> GDPIADMIDQTVNNQVNRSLTALQVLPTAANTEASSHRLGTGVVPALQAAETGASSNASDKNLIETRCVLNHHSTQETAIGNFFSRAGLVSIITMPTTGTQNTDGYVNWDIDLMGYAQLRRKCELFTYMRFDAEFTFVVAKPNGELVPQLLQYMYVPPGAPKPTSRDSFAWQTATNPSV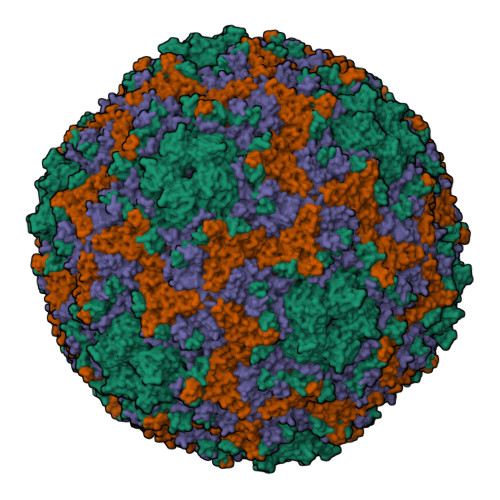FVKMTDPPAQVSVPFMSPASAYQWFYDGYPTFGEHLQANDLDYGQCPNNMMGTFSIRTVGIEKSPHSITLRVYMRIKHVRAWIPRPLRNQPYLFKTNPNYKGNDIKCTSTSRDKITTL;> SPSAEACGYSDRVAQLTIGNSTITTQEAANIVIAYGEWPEYCPDTDATAVDKPTRPDVSVNRFFTLDTKSWAKDSKGWYWKFPDVLTEVGVFGQNAQFHYLYRSGFCVHVQCNASKFHQGALLVAVLPEYVLGTIAGGTGNENSHPPYATTQPGQVGAVLTHPYVLDAGIPLSQLTVCPHQWINLRTNNCATIIVPYMNTVPFDSALNHCNFGLLVIPVVPLDFNTGATSEIPITVTIAPMCAEFAGLRQAVKQ;> GIPTELKPGTNQFLTTDDGVSAPILPGFHPTPPIHIPGEVHNLLEICRVETILEVNNLKTNETTPMQRLCFPVSVQSKTGELCAAFRADPGRDGPWQSTILGQLCRYYTQWSGSLEVTFMFAGSFMATGKMLIAYTPPGGNVPADRITAMLGTHVIWDFGLQSSVTLVVPWISNTHYRAHARAGYFDYYTTGIITIWYQTNYVVPIGAPTTAYIVALAAAQDNFTMKLCKDTEDIEQTANIQ;> MGSQVSTQRSGSHENSNSASEGSTINYTTINYYKDAYAASAGRQDMSQDPKKFTDPVMDVIHEMAPPLK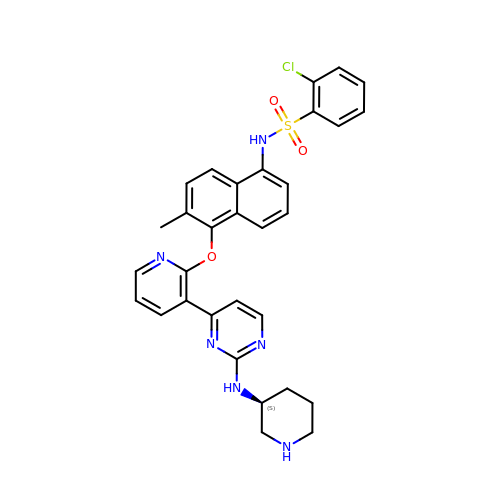2-chloro-N-(6-methyl-5-{[3-(2-{[(3S)-piperidin-3-yl]amino}pyrimidin-4-yl)pyridin-2-yl]oxy}naphthalen-1-yl)benzene-1-sulfonamide | C31 H29 Cl N6 O3 S | XMWUCMFVDXDRDE-NRFANRHFSA-N> SPTVEACGYSD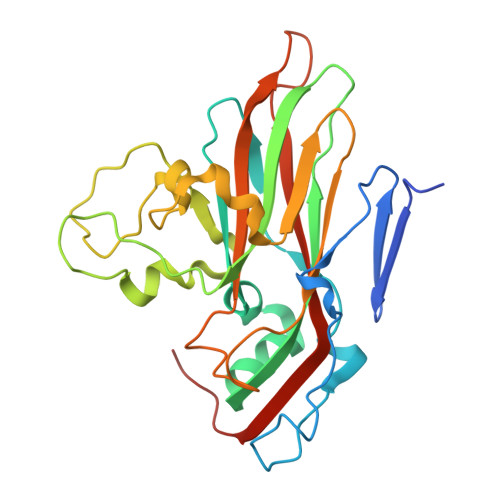RLIQITRGDSTITSQDTANAVVAYGVWPSYLTPDDATAIDKPTQPDTSSNRFYTLDSRSWTSASSGWWWKLPDALKNMGIFGENMFYHFLGRSGYTIHVQCNSSKFHQGLLIVAAIPEHQLASATSGNVSVGYNHTHPGEQGREVVPSRTSSDNKRPSDDSWLNFDGTLLGNLPIYPHQYINLRTNNSATLILPYVNAVPMDSMLRHNNWSLVIIPICPLQVQPGGTQSIPITVSISPMFSEFSGPRSKVVFSTTQ> MRVNNGLTPQELEAYGISDVHDIVYNPSYDLLYQEELDPSLTGYERGVLTNLGAVAVDTGIFTGRSPKDKYIVRDDTTRDTFWWADKGKGKNDNKPLSPETWQHLKGLVTRQLSGKRLFVVDAFCGANPDTRLSVRFITEVAWQAHFVKNMFIRPSDEELAGFKPDFIVMNGAKCTNPQWKEQGLNSENFVAFNLTERMQLIGGTWYGGEMKKGMFSMMNYLLPLKGIASMHCSANVGEKGDVAVFFGLSGTGKTTLSTDPKRRLIGDDEHGWDDDGVFNFEGGCYAKTIKLSKEAEPEIYNAIRRDALLENVTVREDGTIDFDDGSKTENTRVSYPIYHIDNIVKPVSKAGHATKVIFLTADAFGVLPPVSRLTADQTQYHFLSGFTAKLAGTERGITEPTPTFSACFGAAFLSLHPTQYAEVLVKRMQAAGAQAYLVNTGWNGTGKRISIKDTRAIIDAILNGSLDNAETFTLPMFNL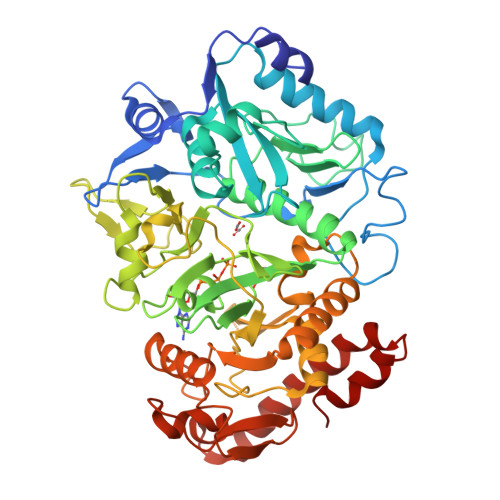AIPTELPGVDTKILDPRNTYASPEQWQEKAETLAKLFIDNFDKYTDTPAGAALVAAGPKL>MDESLEHQTQTHDQESEIVTEGSAVVHSEPSQEGNVPPKVDSEAEVLDEKVSKQIIKEGHGSKPSKYSTCFLHYRAWTKNSQHKFEDTWHEQQPIELVLGKEKKELAGLAIGVASMKSGERALVHVGWELAYGKEGNFSFPNVPPMADLLYEV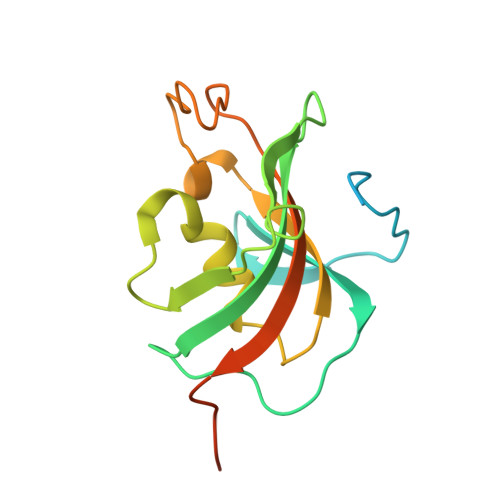EVIGFDETKEGKARSDMTVEERIGAAD[2x]>MSDSHHKPVWDRTHHAKMATGIGDPQCFKGMAGKSKFNVGDRVRIKDLPDLFYTRTMTYTRGATGTIVRLVYESPAAEDEAFGNEENVEWFYSIVFAQKDLWPEYSDTFANDTLETEIPERYLEKA[8x];>[8x]MSSSIREEVHRHLGTVALMQPALHQQTHAPAPTEITHTLFRAYTRVPHDVGGEADVPIEYHEKEEEIWELNTFATCECLAWRGVWTAEERRRKQNCDVGQTVYLGMPYYGRWLLTAARILVDKQFVTLTELHNKIVEMRERVASGQGLGEYLPPKAK;>MSADHDHDHDHDHDHKPAPMVEEVSDFEILEMAVRELAIEKGLFSAEDHRVWKDYVHTLGPLPAARLVAKAWLDPEYKKLCIEDGVEASKAVGVNWVTSPPTQFGTPSDYCNLRVLADSPTLKHVVVCTLCSCYPRPILGQSPEWYRSPNYRRRLVRWPRQVLAEFGLQLPSEVQIRVADSNQKTRYIVMPVRPEGTDGWTEDQLA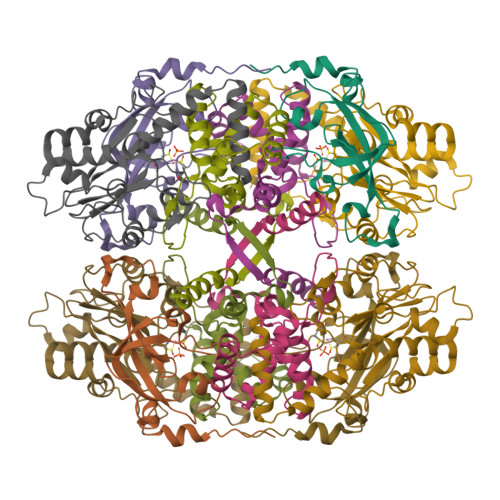EIVTRDCLIGVAVPKPGITVNAKRPVLKANRPVHHDH[8x]>LHFDETGAYTDTSIDTVNKDIVTTRSNLYKKYNQVYDRSAQSFEHVDHYLTAESWYRPKYILKDGKTWTQSTEKDFRPLLMTWWPSQETQRQYVNYMNAQLGINKTYDDTSNQLQLNIAAATIQAKIEAKITTLKNTDWLRQTISAFVKTQSAWNSDSEKPFDDHLQNGAVLYDNEGKLTPYANSNYRILNRTPTNQTGKKDPRYTADNTIGGYEFLLANDVDNSNPVVQAEQLNWLHFLMNFGNIYANDPDANFDSIRVDAVDNVDADLLQIAGDYLKAAKGIHKNDKAANDHLSILEAWSDNDTPYLHDDGDNMINMDNKLRLSLLFSLAKPLNQRSGMNPLITNSLVNRTDDNAETAAVPSYSFIRAHDSEVQDLIRDIIKAEINPNVVGYSFTMEEIKKAFEIYNKDLLATEKKYTHYNTALSYALLLTNKSSVPRVYYGDMFTDDGQYMAHKTINYEAIETLLKARIKYVSGGQAMRNQQVGNSEIITSVRYGKGALKATDTGDRTTRTSGVAVIEGNNPSLRLKASDRVVVNMGAAHKNQAYRPLLLTTDNGIKAYHSDQEAAGLVRYTNDRGELIFTAADIKGYANPQVSGYLGVWVPVGAAADQDVRVAASTAPSTDGKSVHQNAALDSRVMFEGFSNFQAFATKKEEYTNVVIAKNVDKFAEWGVTDFEMAPQYVSSTDGSFLDSVIQNGYAFTDRYDLGISKPNKYGTADDLVKAIKALHSKGIKVMADWVPDQMYAFPEKEVVTATRVDKFGKPVEGSQIKSVLYVADSKSSGKDQQAKYGGAFLEELQAKYPELFARKQISTGVPMDPSVKIKQWSAKYFNGTNILGRGAGYVLKDQATNTYFNISDNKLEHHHHHH[2x]

Streptococcus mutans employs a key virulence factor, three glucosyltransferase (GtfBCD) enzymes to establish cariogenic biofilms. While GtfB synthesizes pre-dominantly insoluble glucans, GtfD only produces water-soluble glucans, and GtfC can synthesize both soluble and insoluble glucans. All Gtfs are composed of three functional regions: the N-terminal variable junction region, the C-terminal glucan-binding region, and the highly conserved catalytic region in the middle, which is essential for the glucan synthesis. Previous studies have demonstrated that glucans produced by GtfB and GtfC are essential for the assembly of the S. mutans biofilms, while glucans produced by GtfD serve not only as a primer for GtfB, but also as a source of nutrient for S. mutans and other bacteria.

Seven potent biofilm inhibitors emerged from this study, the lead compound #G43 was further characterized and shown to have anti-biofilm activity through the binding to GtfBC and the inhibition of the activity of GtfBC. Compound #G43 consistently inhibited the activity of both GtfB and GtfC, ImageJ analysis of the intensities suggest 80% inhibition of both enzymes, while compound #G16 had a smaller effect on the activity of GtfB (60% inhibition) and GtfC (70% inhibition). To determine if the inhibition is attributed by the binding of the lead compound to the enzymes, the OctetRed96 system was used to characterize protein-small molecule binding kinetics. The his-tagged catalytic domains of GtfB and GtC were immobilized separately onto an anti-penta-HIS (HIS1K) biosensor which consists of high affinity, high specificity penta-his antibody pre-immobilized on a fiber optic biosensor. This sensor was then exposed to varying concentrations of #G43. Assay data fit to a 1:1 binding model with a fixed maximum response, which produced a KD value of 3.7 µM for GtfB. The KD value for GtfC was more potent at 46.9 nM. As the catalytic domain of GtfB and GtfC shares 96% similarity at amino acid sequence level, the selectivity by the compound is remarkable. Binding studies of this analog against GtfB yielded a KD value of 68 µM, compared to a KD value of 3.7 µM by the active analog. An analog that does not contain this functional group lost the ability to inhibit the activity of Gtfs and in vitro biofilm formation, demonstrating that these effects are directly related and that the inclusion of the primary ortho amide group is crucial to maintaining potent anti-biofilm activity.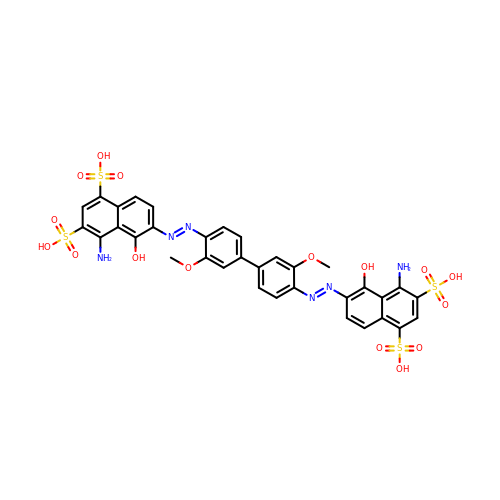6,6'-[(3,3'-dimethoxybiphenyl-4,4'-diyl)di(E)diazene-2,1-diyl]bis(4-amino-5-hydroxynaphthalene-1,3-disulfonic acid) | C34 H28 N6 O16 S4 | OHMJKMNGYYWCHB-HVMBLDELSA-N> ASRSQAEDVRVEGSFPVTMLPGDGVGPELMHAVKEVFKAAAVPVEFQEHHLSEVQNMASEEKLEQVLSSMKENKVAIIGKIHTPMEYKGELASYDMRLRRKLDLFANVVHVKSLPGYMTRHNNLDLVIIREQTEGEYSSLEHESARGVIECLKIVTRAKSQRIAKFAFDYATKKGRGKVTAVHKANIMKLGDGLFLQCCEEVAELYPKIKFETMIIDNCCMQLVQNPYQFDVLVMPNLYGNIIDNLAAGLVGGAGVVPGESYSAEYAVFETGARHPFAQAVGRNIANPTAMLLSASNMLRHLNLEYHSSMIADAVKKVI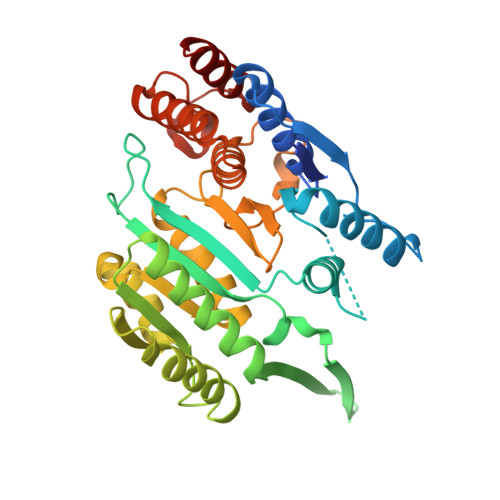KVGKVRTSDMGGYATCHDFTEEICRRVKDLDEN>[2x]SKRIEKRTKFTVDDHVVAWKFIYEKLVEADKEGVQLMPKGIAFWNDFVRVTRSSKSATNWSSHFRKIMCPGLHEMPLH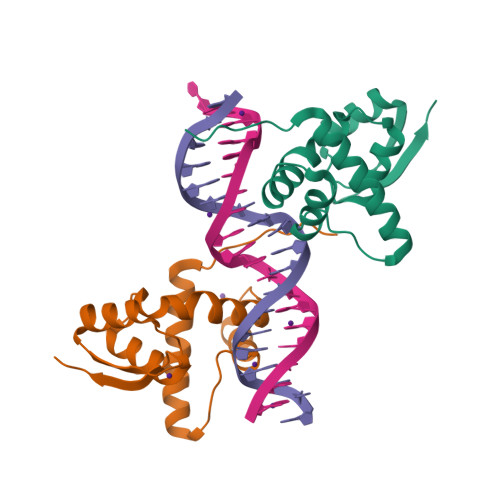KKTILYLLKNIGIEIDKETEQIIERKFNVKLLVGIDRNLISYKLLDA>[4x]TQDCSFQHSPISSDFAVKIRELSDYLLQDYPVTVASNLQDDELCGG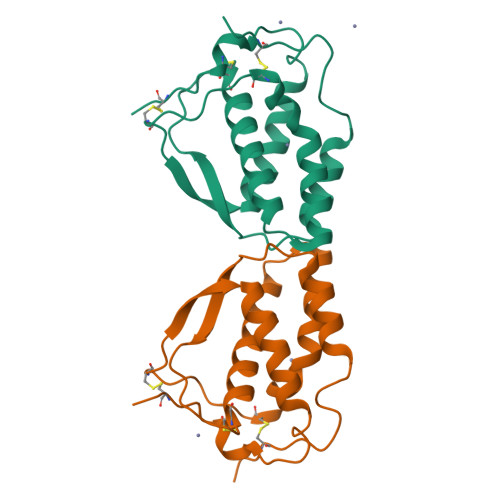LWRLVLAQRWMERLKTVAGSKMQGLLERVNTEIHFVTKCAFQPPPSCLRFVQTNISRLLQETSEQLVALKPWITRQNFSRCLELQCQP> AFNNNPSSVGAYSSGTYRNLAQEMGKTNIQQKVNSTFDNMFGYNNTQQLYYPYTENGVYKAHYIKAINPDEGDDIRTEGQSWGMTAAVMLNKQEEFDNLWRFAKAYQKNPDNHPDAKKQGVYAWKLKLNQNGFVYKVDEGPAPAGEEYFAFALLNASARWGNSG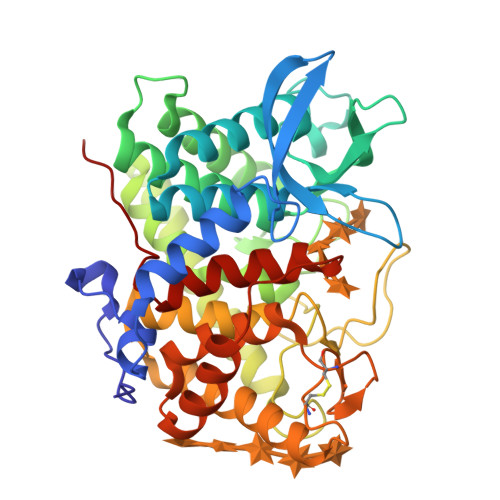EFNYYNDAITMLNTIKNKLMENQIIRFSPYIDNLTDPSYHIPAFYDYFANNVTNQADKNYWRQVATKSRTLLKNHFTKVSGSPHWNLPTFLSRLDGSPVIGYIFNGQANPGQWYEFDAWRVIMNVGLDAHLMGAQAWHKSAVNKALGFLSYAKTNNSKNCYEQVYSYGGAQNRGCAGEGQKAANAVALLASTNAGQANEFFNEFWSLSQPTGDYRYYNGSLYMLAMLHVSGNFKFYNNTFN> 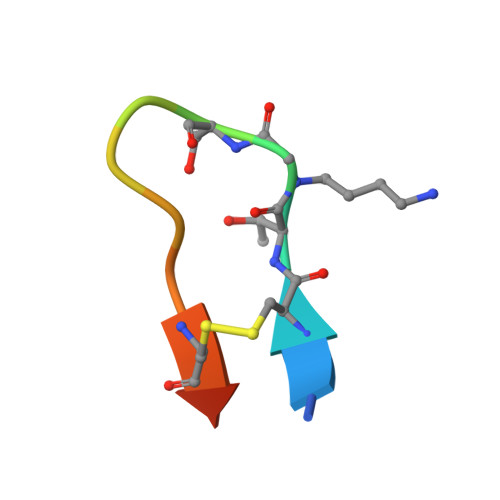GRCTXSIPPICFPD>[2x]MENTENSVDSKSIKNLEPKIIHGSESMDSGISLDNSYKMDYPEMGLCIIINNKNFHKSTGMTSRSGTDVDAANLRETFRNLKYEVRNKNDLTREEIVELMRDVSKEDHSKRSSFVCVLLSHGEEGIIFGTNGPVD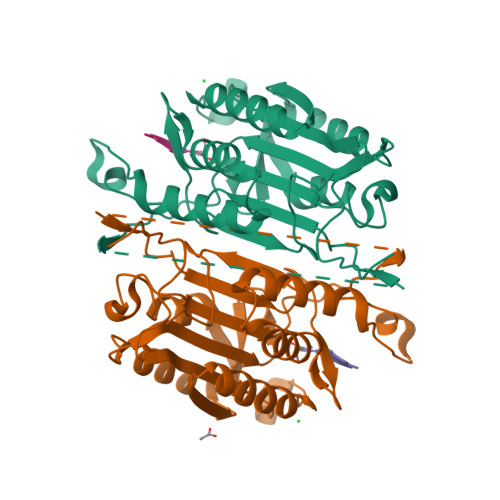LKKITNFFRGDRCRSLTGKPKLFIIQACRGTELDCGIETDSGVDDDMACHKIPVEADFLYAYSTAPGYYSWRNSKDGSWFIQSLCAMLKQYADKLEFMHILTRVNRKVATEFESFSFDATFHAKKQIPCIFSMLTKELYFYHLH>[2x]MSTTIQYNSNYADYSISSYLREWANNFGDIDQAPAETKDRGSFSGSSTLFSGTQYAIGSSHSNPEGMIAEGDLKYSFMPQHTFHGQIDTLQFGKDLATNAGGPSAGKHLE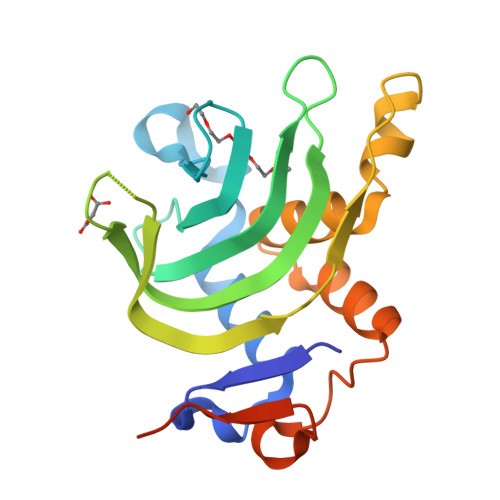KIDITFNELDLSGEFDSGKSMTENHQGDMHKSVRGLMKGNPDPMLEVMKAKGINVDTAFKDLSIASQYPDSGYMSDAPMVDTV>SNVLDGLKYAPSHEWVKHEGSVATIGITDHAQDHLGEVVFVELPEPGVSVTKGKGFGAVESVKATSDVNSPISGEVIEVNTGLTGKPGLINSSPYEDGWMIKIKPTSPDELESLLGAKEYTKFCEEED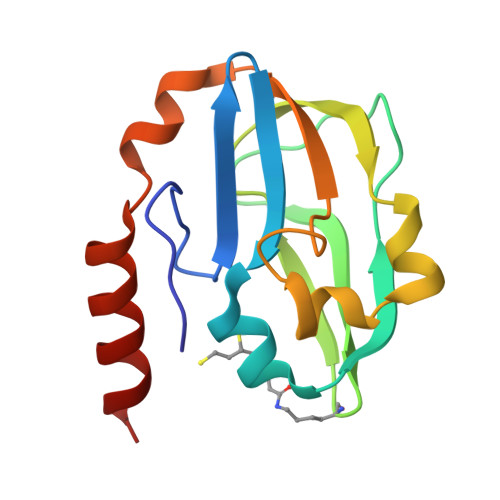AAH[2x]> GGCUUAUCAAGAGAGGUGGAGGGACUGGCCCGAUGAAACCCGGCAGCC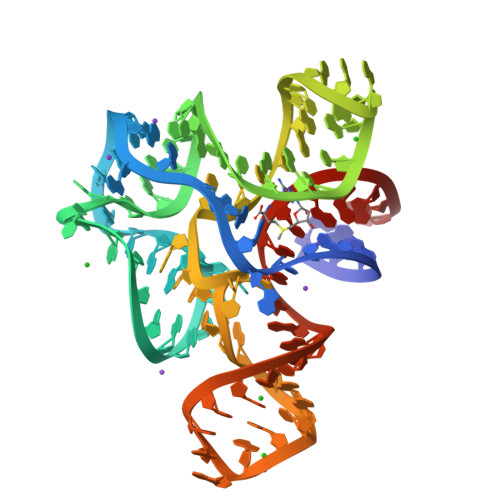AGAAAUGGUGCCAAUUCCUGCAGCGGAAACGUUGAAAGAUGAGCCG>[2x]GNEDDVMEIFNDKTWKLSRITTEKGKEQFY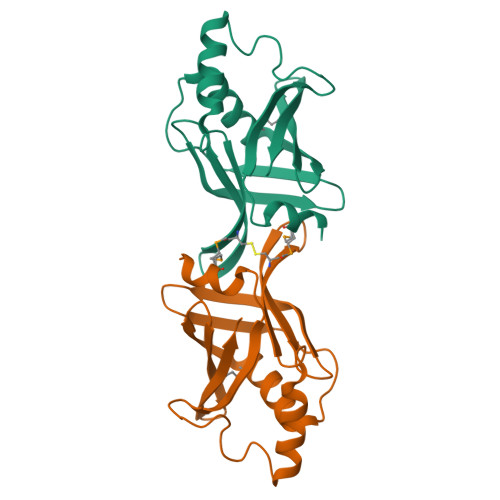QGLWSNEAEEKASRELLKITENFTLNFNCADVNGEVTGTVSAHAVKANISDAILKIDGKEHTISISGKAYGSESDKLAKVFISGLFNVFKYEGDVHNLTLYFKDGNTTKVMGFTAR>[2x]MIERRKIAVIGSGQIGGNIAYIVGKDNLADVVLFDIAEGIPQGKALDITHSMVMFGSTSKVIGTNDYADISGSDVVIITASIPGRPKDDRSELLFGNARILDSVAEGVKKYCPNAFVICITNPLDVMVSHFQKVSGLPHNKVCGMAGVLDSSRFRTFIAQHFGVNA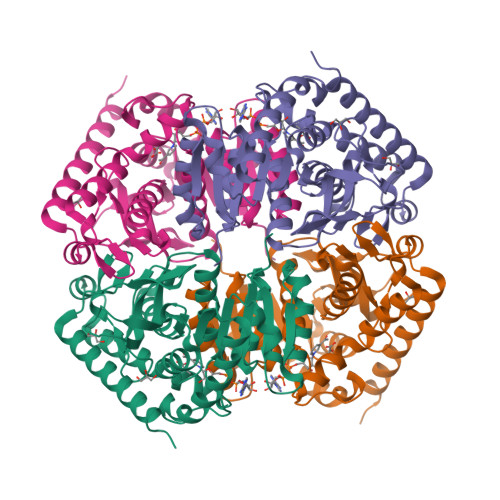SDVSANVIGGHGDGMVPATSSVSVGGVPLSSFIKQGLITQEQIDEIVCHTRIAWKEVADNLKTGTAYFAPAAAAVKMAEAYLKDKKAVVPCSAFCSNHYGVKGIYMGVPTIIGKNGVEDILELDLTPLEQKLLGESINEVNTISKVLDNAPAAGA>[2x]MPYDHNAEADFAASEVARMLVADPGLCYDAASLPASISASASYEPSAAGWPKADGLVSVLEGGTSTQRAIALEYKRPQEGIHGLLTAIGQAHGYLHKGYSGAAIVIPGRYSSHPTPAEYVRDVLNAISGSRAIAVFSYSPPDTTSPTPFAGRIQCVRPLVFDAGRVHLRPANQGPKTQWVHMREGSTTRDAFFRFLQVAKRLSADPTAPRPTLRSELVAAIGRLAPGRDPIEYITNTADNKFLTKVWQFFWLEWLATPA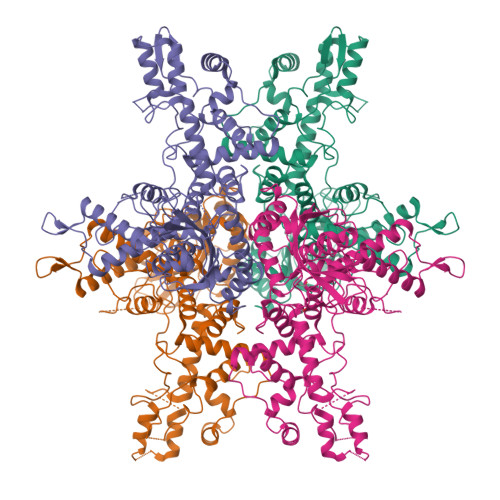VLTPWKLEAGVYSAPGARTRILREDGTDFSQLWEGRVNSLKETIAGMLNRGEISEAQGWEAFVGGISATGGGQDKQGVRARAHSYREDIDSALAQLRWIEDDGLPTDQGYRFMTICERYGGANSRAAIDYMGATLIQTGRYASFLHYINRLSERKFAENPLAYTKPGPGGMPVFTEESYWEYLQDLETKLTDELRVMRKVSGRARPRVRTTFQVELTLLRNYGFVSSTRHRLGVGIPIDWEQVVQALNVDL> MGGDLKVKMLGGEEILVPLRDSMMVSELKQFIAQKINVPAFQQRLAHL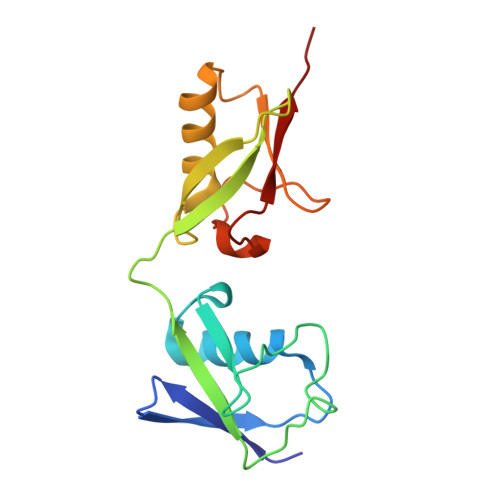DSREVLQEGVPLVHQGLKAGSTILLMVQNSSATLNILVRNDKGRSSSYEVQLTQTVAVLKQQVCQRERVQADQFWLSFEGKPMDDEHPLGEYGLTTGCTVFMNLRLRG PB28 | C24 H38 N2 O | 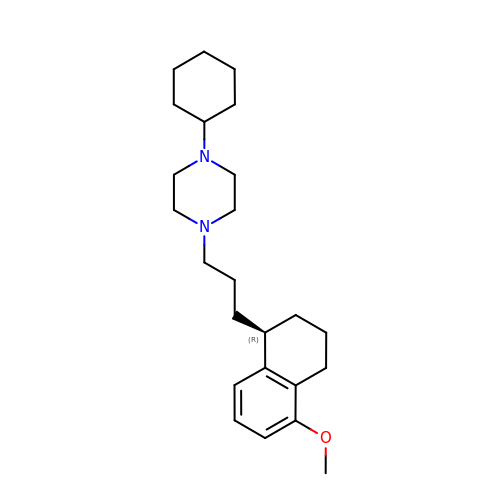PHRCDWVPTULQMT-HXUWFJFHSA-N>[8x]MNIGVIILAAGEGKRFGGDKLLAKIDNTPIIMRTIRIYGDLEKIIIVGKYVNEMLPLLMDQIVIYNPFWNEGISTSLKLGLRFFKDYDAVLVALGDMPFVTKEDVNKIINTFKPNCKAVIPT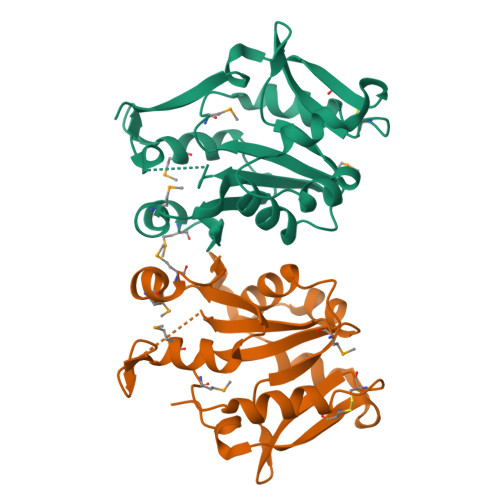HKGERGNPVLISKSLFNEIEKLRGDVGARVILNKIKIEELCFIECSEGVLIDIDKKEDLMRLRDFHPLEHHHHHH> MYKILEKKEIAMRNTWYKVYAPHVAKKVQPGQFVIVRAFP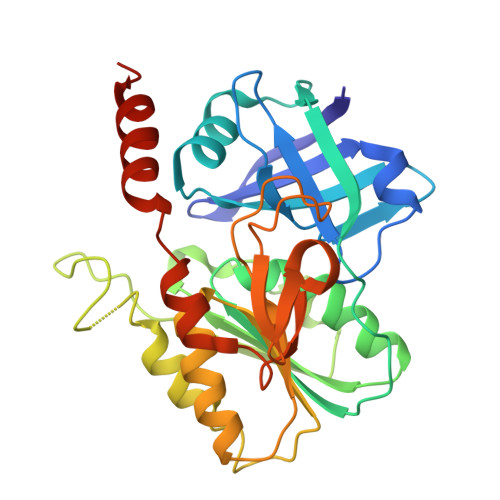NGERIPLTPVMWDREEGWIVLIVFTRGKTTMRMAVELKEGDSLLNVAGPLGTPVPMEKFGKILAIGAYTGIVEVYPIAKAWQEIGNDVTTLHVTFEPMVILKEELEKAVTRHIVEPVPLNPNQDFLANMKNVSQRLKEKVRELLESEDWDLVFMVGPVGDQKQVFEVVKEYGVPMKVDLHPIMVDGTGMCGACRVTVGGEVKFACVDGPEFDAYQVDWDELIHRVGFYAKLEKLALEKYMEELKAKGVI>[2x]GPGSEFQRPTMESVRNFEQWQSQRNQLQGAMQQFNQRYLYSASMLAAENDPYGPLPPGWEKRVDSTDRVYFVNHNTKTTQWEDPRTQGLQNEEPLPEGWEIRYTREGVRYFVDHNTRTTTFKDPRNGKSSVTKGGPQIAYERGFRWKLAHFRYLCQSNALPSHVKINVSRQTLFEDSFQQIMALKPYDLRRRLYVIFRGEEGLDYGGLAREWFFLLSHEVLNPMYCLFEYAGKNNYCLQINPASTINPDHLSYFCFIGRFIAMALFHGKFIDTGFSLPFYKRMLSKKLTIKDLESIDTEFYNSLIWIRDNNIEECGLEMYFSVDMEILGKVTSHDLKLGGSNILVTEENKDEYIGLMTEWRFSRGVQEQTKAFLDGFNEVVPLQWLQYFDEKELEVMLCGMQEVDLADWQRNTVYRHYTRNSKQIIWFWQFVKETDNEVRMRLLQFVTGTCRLPLGGFAELMGSNGPQKFCIEKVGKDTWLPRSHTCFNRLDLPPYKSYEQLKEKLLFAIEETEGFGQE

The Nedd4 family E3s have nine members in humans (WWP1/2, Nedd4/4 L, Smurf1/2, NEDL1/2, and Itch), which share a common N-terminal domain architecture comprised of a C2 domain and 2–4 WW domains that are responsible for subcellular localization and substrate recognition, respectively. Each HECT-type E3 contains a characteristic HECT domain at its C terminus, which catalyzes the transfer of ubiquitin from E2 to itself and then to the specific substrate. The HECT domain adopts a bilobal structure, in which the E2-binding N-lobe is connected by a flexible hinge loop to the catalytic C-lobe. To prevent excessive ubiquitination of targets and self-destruction by autoubiquitination, HECT-type E3s normally adopt an inactive state characterized by intra- or inter-molecular interaction.

To elucidate the molecular mechanism governing WWP1 autoinhibition, we determined the crystal structures of WWP1 in its fully inactive (2L34HECT) and partially active (L34HECT) states at resolutions of 2.3 Å and 2.5 Å, respectively. In contrast, the presence of the adjacent WW domain(s) together with L (e.g., 2LHECT or L34HECT) led to dramatic decreases in WWP1 autoubiquitination, suggesting that both WW2 and WW34 are responsible for ligase regulation. Both 2LHECT and L34HECT mutants possess slightly elevated ligase activity compared to 2L34HECT, indicating that they adopt a partially active state. In the L34HECT crystal structure, WW3, WW4, and the entire L region were well-resolved. It seems that the WW3 and WW4 domains are packed closely together, WW4 binds to the same “Le” site on HECT, and L forms a kinked α-helix that resides at the same “H” site that spans from the “Re” site to the “Le” site. Compared with 2L34HECT, WW4 and the N-terminal part of L are rotated ~35 and 25 degrees, respectively in L34HECT, and a few N-terminal residues (aa 413–416) in L were not observed. Importantly, although the 35 degree rotation of WW4 and 25 degree rotation of L appear to be significant, the crucial WW4-HECT and L-HECT contacts in the 2L34HECT structure are preserved in L34HECT. Our assumption is that the WW4-binding N-terminal extension of HECT is a flexible loop, which allows HECT-bound WW4 to rotate a certain extent upon crystal packing with a symmetric molecule in 2L34HECT; whereas the 25 degree rotation of the N-terminal part of L is the result of the missing WW2 domain and crystal contacts. We further validated the functional relevance of the WW4-HECT interaction in L34HECT. The point mutation at the WW4-HECT-binding surface (H517AWW4 or Y543AHECT) severely impaired the WW4-HECT interaction. Meanwhile, mutations at the WW4-HECT packing interface in WW4 (E503A, H517A, and H517Y) or HECT (Y543A, Y543E, W549A) led to significantly elevated autoubiquitination of WWP1 L34HECT, further demonstrating that the crystal packing-induced rotation of WW4 does not affect its inhibition in HECT activity.>[2x]IDPKDLTFLKELGTGQFGVVKYGKWRGQYDVAIKMIKEGSMSEDEFIEEAKVMMNLSHEKLVQLYGVCTKQRPIFIITEYMANGCLLNYLREMRHRFQTQQLLEMCKDVCEAMEYLESKQFLHRDLAARNCLVNDQGVVKVSDFGLSRYVLDDEYTSSVGSKFPVRWSPPEVLMYSKFSSKSDIWAFGVLMWEIYSLGKMPYERFTNSETAEHIAQGLRLYRPHLASEKVYTIMYSCW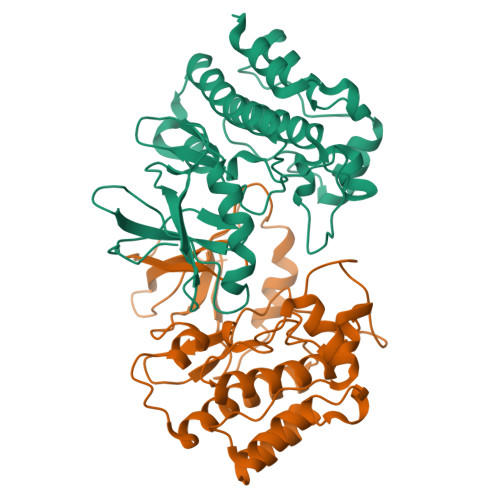HEKADERPTFKILLSNILDVMDEES In this article, we studied five members of the PLL lectin family from P. laumondii subsp. laumondii TT01 (PLL, PLL2, PLL3, PLL4, PLL5, collectively referred to as PLLs). All studied lectins belong to the seven-bladed β-propeller structural family. Each blade makes a W-motif composed of four antiparallel beta-strands (β1-β4) connected by β-turns and loops. The saccharide binding sites are located between the adjacent blades and are uniquely organized in two separate circles around the monomer.

The PLL chain A blade W1 interacts with chain B blade W3, whereas in the case of PLL2, PLL4 and PLL5, chain A blade W1 interacts with chain B blade W5. The highest affinity was seen towards methyl-α-l-fucoside (αMeFuc), ranging from 0.4 ± 0.02 mM for PLL2 to 4.9 ± 0.08 mM for PLL4. l-fucose was also significantly recognized. In this study, we confirmed that PLL2 highly increased ROS production and discovered that other PLLs also activate a similar oxidative response, suggesting that the immune systems of both humans and insects recognise all these lectins. In human blood activated by zymosan A, PLL2 and PLL3 inhibited ROS production, suggesting these lectins interfere with the innate immune system reaction in the early stages of the Photorhabdus infection. Different behaviour was seen for d-galactose, which inhibited only the binding of PLL3 and not PLL2, despite confirmed binding to both proteins from ITC, suggesting that d-galactose aims for different binding sites than MGMR in PLL2.

>[2x]MQEEPTNIPRPDNAELLVASEVAIENAAIALSEIVSVVNTSDGRIEVFGVGTDNAVWHNRQTAPHSGSSWTGWISLNGKVTSKPVVYINTDGRLEVFARGTDNALWHIWQTATNAGWSNWQSLGGTITSNPAVYVNTDGRIDVFARGTDNALWHISQTAAHSGPWSSWQSLNGVITSNPAVHINSDGRLEVFARGTDNALWHIWQTAPDSNQWSGWDSLGGVITSDPVVIGTADGRLEVFARGSNNALYHIWQTVPHGGPWSNWASLNGVITSAPAVVKNSDGRLEVFARGTNNALYHIWQTVSHSGPWSNWATLNGTITSAPTAVEDADGRLEVFARGTDNALWNIWQATPSWSAWVSLKGSLIDASAIK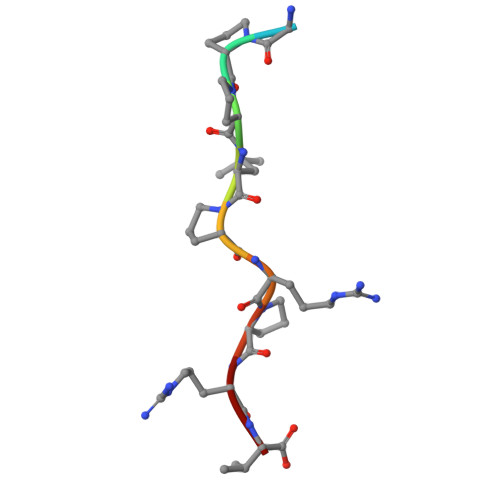> KGPPLPRPRV> NISDYKVMTWNLQGSSASTESKWNVNVRQLLSGTAGVDILMVQEAGAVPTSAVPTGRHIQPFGVGIPIDEYTWNLGTTSRQDIRYIYHSAIDVGARRVNLAIVSRQRADNVYVLRPTTVASRPVIGIGLGNDVFLTAHALASGGPDAAAIVRVTINFFRQPQMRHLSWFLAGDFNRSPDRLENDLMTEHLERVVAVLAPTEPTQIGGGILDYGVIVDRAPYSQRVE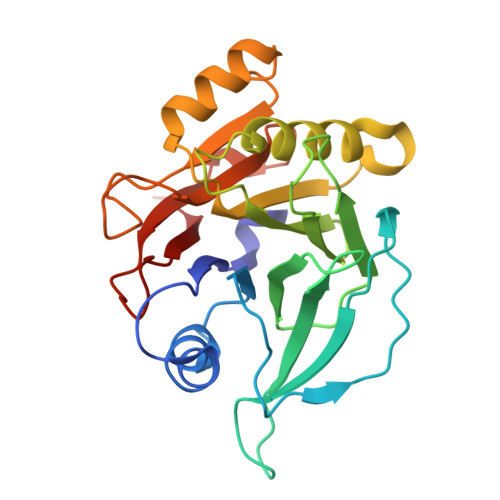ALRNPQLASDHYPVAFLARSCL>[2x]MTAVTLDGGWRVRLVPGQEQGKTYPKAAAWLPAQVPGAVQTDLIAAKIVPDPFYRDNEGKIQWAGLSDWQYQTRFTVDAATLKREHVELVFDGLDTFAEVTLNGKQLLSADNMFRQWRVDAKSLLKRGDNLLEVKLYSPIKKIQPWLAKQPYALPGAYDSAFGDEPEARHSSTYVRKAPYNFGWDWGPRMVNAGIWKDVRVEAWDAVRVDGLHIAQQRVDAHSAQVQAQLDLQAGRSGPVQVTLDVLGPDGQKVGQFTQDAVVDPGQNRVDLAVRIANPKRWFPAGYGAQDRYTFVASVRDADGDSQQIKRV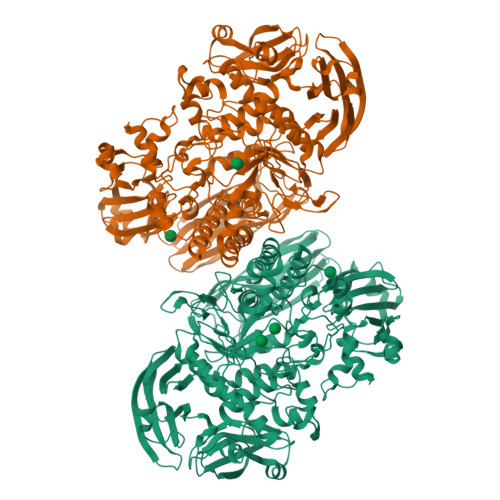TGLRSVELRREKDRFGKSMEIVINGIPIFAKGANLIPLDAFPARVTHERMRSTLQDARDANMNMLRMWGGGHYQDDYFYDVADELGIMIWQDFMFGGAVPPYDVEFRENTRQEAIEQVKRLRDHPSLVLWCGNNAVQTGWENWGDRVKFKQSVDPEERTRIERGMTTLFGTVFREVVATYDSDVPYWATSPGTDFDGAADQTNDGDMHYWKVWGGPALPVTEYLNVTPRFMSEYGLQSFPDMRTVRAFAEPGDMDPESPVMRVHQKFDKGNGNKRLMLYIRREFGEPKDFESFVYLSQLMQAEGINIAASHLRASRPQSMGSLYWQLNDVWPGASWSSVDYYGRWKALHYHARRFYAPEMIAALRNDKGQTEVSLVSDRTTPLTARWRMRVMGMDGKVLSKREEKASVNALSSQHVGNFSDKQLLGSADPKRTYAVFELLDGDTLLSREVVFFAPAKQLALPAAKIDSQWRADGDGYALTLTSDTLAREVWLSFGDVDATLSDNAFDLLPGEPLTVRVTSKAALAQLQSALQVRDLAATLAGAPPEP> APIRY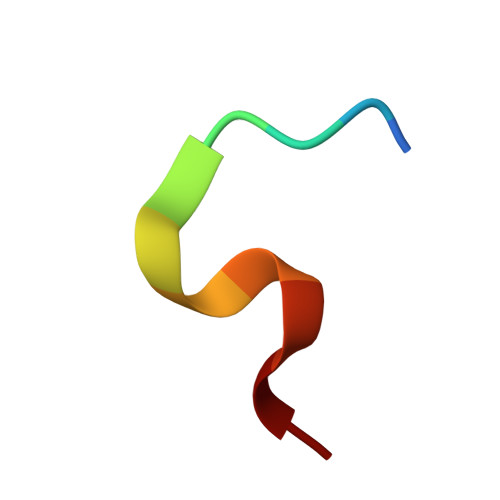EWDEFC>MNHKVHHHHHHIEGRHMKVNISIFGFGTVGRALAEIIAEKSRIFGVELNVISITDRSGTIWGDFDLLEAKEVAESTGKLSNIGDYEVYNFSPQELVEEVKPNILVDVSSWDEAHEMYKVALGEGISVVTSNKPPIANYYDELMNLAKENNAGIFFESTVMAGTPIIGVLRENLLGENIKRIDAVVNASTTFILTKMSEGKTLDDAIEEAKSLGILEEDPSKDIDGI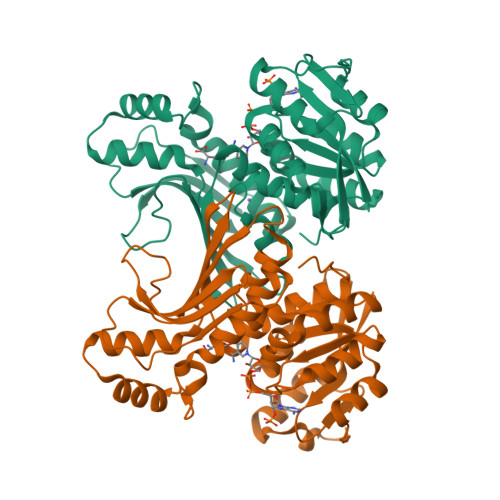DAYYKAKILHWVSYGEPPEEEERLGIREVRDARNVRLVAQVSKGKISVKPRKLSSDNPLLVEGVQNAAVIRTNNLGEVILKGPGGGGRVTASGVFTDIIKATLKFPNLR[2x]>MQWSGARALEALLTVAGELRGPPLQLDTGQLLKIAKRGGVTAVEAVHAWRNALTGAPLNLTPEQVVAIASHDGGKQALETVQRLLPVLCQAHGLTPQQVVAIASHDGGKQALETVQRLLPVLCQAHGLTPEQVVAIASHDGGKQALETVQALLPVLCQAHGLTPEQVVAIASNGGGKQALETVQRLLPVLCQAHGLTPQQVVAIASNGGGKQALETVQRLLPVLCQAHGLTPQQVVAIASNGGGKQALETVQRLLPVLCQAHGLTPQQVVAIASNNGGKQALETVQRLLPVLCQAHGLTPQQVVAIASNGGGKQALETVQRLLPVLCQAHGLTPQQVVAIASHDGGKQALETVQRLLPVLCQAHGLTPEQVVAIASNGGGKQALETVQRLLPVLCQAHGLTPEQVVAIASHDGGKQALETVQRLLPVLCQAHGLTPQQVVAIASNGGGRPALESIVAQLSRPDPALAALTNDHLVALACLGGRPALDAVKKLEHHHHHH[2x]

Transcription activator-like (TAL) effectors specifically bind to double stranded (ds) DNA through a central domain of tandem repeats. Each TAL effector (TALE) repeat comprises 33–35 amino acids and recognizes one specific DNA base through a highly variable residue at a fixed position in the repeat. The crystal structures of TAL effector (TALE) proteins bound to their respective target DNAs have revealed that the residue at position 13 is the only one directly involved in DNA base recognition, whereas the 12th residue stabilizes the proper loop conformation. dHax3, an engineered TALE protein, proved to be a useful scaffold for structural characterizations. We then present fifteen crystal structures of engineered dHax3 variants in complex with target DNA molecules, which elucidate the structural basis for the recognition of bases adenine (A) and guanine (G) by reported or uncharacterized TALE codes.

To test this speculation, we generated dHax3 variants with the 34th residue on repeat 7 substituted with different amino acids. In total, we obtained nine high-quality structures that elucidate the accommodation of base A by Leu, Met, Cys, Pro, Trp, His, Thr, Asn, and Glu at the 34th position. On the other hand, Asn34 and Glu34 can both be H-bonded to base A, although the recognition between Glu34 and base A was unreported previously. Interestingly, the side group of Asn34 donates an H-bond to N7 atom of A, reminiscent of what was seen for the coordination of base G in the DNA-bound PthXo1 structure. Asn34 form the hydrogen bond in a different way with both A and G. The length of the hydrogen bonds are about 3 Å. Given that O6 atom in base G is more electronegative than N7 atom in base A, the H-bond with O6 atom may represent a stronger interaction. On the other hand, Asn34 was originally thought to be a strong code for both G and A. Recent study indicated that Asn34 favors G over A when a large number of these bases exist within a given sequence. Asn34 is a strong code for base A only when the discrimination between A and G is not a concern with the target DNA sequences. Nevertheless, the discriminative binding of A and G by Asn34 or His34 unveiled by the structures provide unprecedented clarity to understand the biochemical observations.> PNFSGNWKIIRSENFEELLKVLGVNVMLRKIAVAAASKPAVEIKQEGDTFYIKVSTTVWTTEIN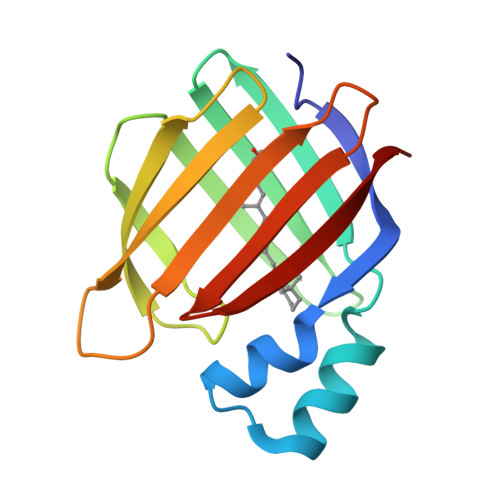FKVGEEFEEQTVDGRPCKSLVKWESENKMVCEQKLLKGEGPKTSWTKELTNDGELILTMTADDVVCTLVFVRE The translocase of the outer membrane (TOM) is the main protein-import pore of mitochondria, recognizing nascent precursors of mitochondrially targeted proteins and transferring them across the outer membrane. TOM core complexes are membrane-embedded stoichiometric complexes with two pores, each containing five subunits: Tom40, Tom22, Tom7, Tom6 and Tom5. The main component of TOM is its translocation pore, Tom40, which is closely related to the mitochondrial porins (voltage-dependent anion channels; VDACs; Pusnik et al., 2009); the 19-strand β-barrel has an internal α-helix (α2) that limits the size of the pore. The small TOM subunits Tom5, Tom6 and Tom7 are membrane-embedded single α-helices that adopt characteristic shapes and interface with the outer surface of Tom40, shielding regions that are exposed to the cytosol.

A 3.3 Å resolution map and molecular model of a TOM complex from Drosophila melanogaster, obtained by single-particle electron cryomicroscopy, is presented. The core TOM complex extracted from native membranes of the D. melanogaster retina contains transgenic Tom40 co-assembled with four endogenous TOM components: Tom22, Tom5, Tom6 and Tom7. The final model contains all subunits of the core complex, comprising two copies of the 19-stranded β-barrel Tom40, two copies of the precursor receptor subunit Tom22 and two copies each of Tom5, Tom6 and Tom7. The Tom40 model is missing only the disordered N-terminal domain in the intermembrane space, while Tom22 is missing its disordered N- and C-terminal domains. The map resolution was insufficient to identify the lipid headgroups, and thus all were conservatively modeled as phosphatidyl choline (PC), as mass-spectrometric studies of the human TOM complex had indicated that most bound lipids were PC. The two β-barrels are thus mutually inclined at approximately 20°, exhibiting the characteristic chevron-like TOM architecture. Unique to Drosophila Tom40, the proline-rich loop β10–β11 (220GPNVPGR226) points into the interior of the β-barrel. In Saccharomyces the C-terminal helix is present but veers away from the β3–β4 loop in the structure. Both the Drosophila and human Tom40 structures lack a C-terminal helix, terminating at the 19th stave of the barrel [Fig. 5(b)].

>[2x]AALENPGTVEELHKKCKDIQAITFEGAKIMLNKGLSNHFQVSHTINMSNVVPSGYRFGATYVGTKEFSPTEAFPVLLGDIDPAGNLNANVIHQFSARLRCKFASQIQESKVVASQLTTDYRGSDYTLSLTVANPSIFTNSGVVVGQYLQSVTPALALGSELAYQFGPNVPGRQIAIMSVVGRYTAGSSVWSGTLGQSGLHVCYYQKASDQLQIGAEVETSLRMQESVATLAYQIDLPKANLVFRGGIDSNWQIFGVLEKRLAPLPFTLALSGRMNHVKNNFRLGCGLMIG;>[2x]ATVKSVKGFYSFSCNASWIFFTSAVILFAPVIFETERAQMEELHKSQ;>[2x]DRLGFVVGVVQTGFHWGFVPLVLYLGFMKGAEPGMPPLNLFSLLWQ;>[2x]PLSIVRSIYNNEFQWMLVKSYGLFFLGVRLAKEFVGVELMPS;>SQPDPAEEQKRVAAEVRFNFILFGAVIAAVRLAPIVLKH[2x]> GPHMRKKRKDINTIEDAVKLLQECKKIIVLTGAGVSVSCGIPDFRSRDGIYARLAVDFPDLPDPQAMFDIEYFRKDPRPFFKFAKEIYPGQFQPSLCHKFIALSDKEGKLLRNYTQNIDTLEQVAGIQR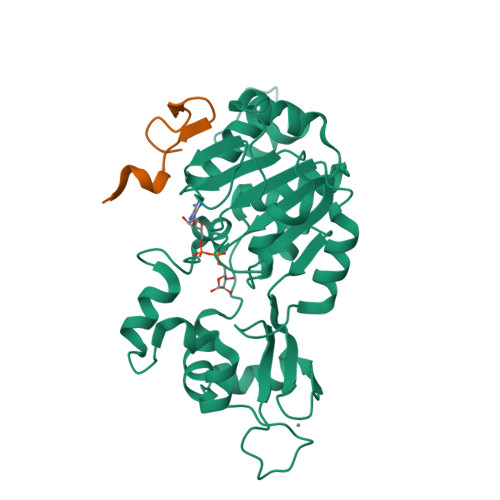IIQCHGSFATASCLICKYKVDCEAVRGDIFNQVVPRCPRCPADEPLAIMKPEIVFFGENLPEQFHRAMKYDKDEVDLLIVIGSSLKVRPVALIPSSIPHEVPQILINREPLPHLHFDVELLGDCDVIINELCHRLGGEYAKLCCNPVKLSEI;> GPHMGSQYLFLPPNRYIFHGAEVYSDSEDDV2-[(5-chloro-2-{[4-(4-methylpiperazin-1-yl)phenyl]amino}pyrimidin-4-yl)amino]phenyl 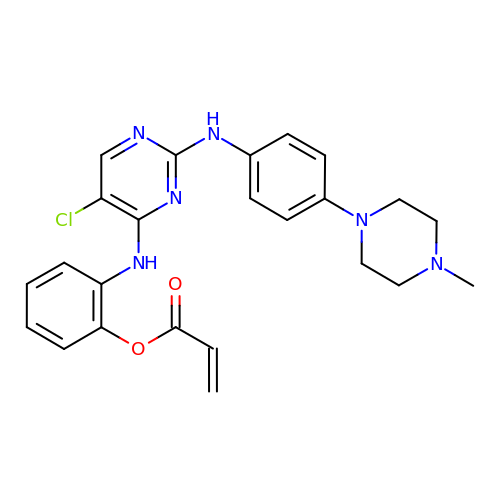prop-2-enoate | C24 H25 Cl N6 O2 | YEUSGXFRXSLYPA-UHFFFAOYSA-N Old Yellow Enzymes (OYEs, EC 1.6.99.1) are a class of flavin-dependent ene-reductases (ERs) catalyzing the asymmetric hydrogenation of electronically activated C=C bonds in the presence of nicotinamide cofactors. We have identified and produced four new putative ERs from the filamentous fungi Aspergillus niger CBS 513.88 and Botryotinia fuckeliana B05.10. Based on the most recent classification, AnOYE2 and BfOYE1 belong to Class II OYEs, as they share all the fingerprint motifs described for “classical” OYE homologues identified in fungi. On the other hand, AnOYE8 and BfOYE4 share most of the typical conserved residues reported in Class III OYEs (S23, P24, C26, A60, Q102, R215, S249, Q265, G284, M285, F305, G307, R308, and R312; YqjM numbering).

AnOYE8 was solved and refined in the C121 space group with four molecules per asymmetric unit. The overall structure of a single subunit showed the typical conserved α8/β8-TIM barrel fold. In agreement with the general behavior of Class III OYEs, the four molecules within the asymmetric unit assembled into dimers with the functional quaternary architecture peculiar of these enzymes. AnOYE8 is an elongated dimer composed of two protomers with an interacting surface of 2807 Å2 (data obtained by EMBL-EBI-PISA analysis). Both the α1-helix and loop 3 (capping subdomain), as well as the peculiar long N-terminal and C-terminal loops of each protomer, were involved in the dimerization surface, which contained 71 interfacing residues that established 18 hydrogen bonds and 8 salt bridges. The C-terminus of each subunit (from Gly393 to Lys416) protruded through an “amino acid finger” (Trp397) that reached the active site of the adjacent subunit, shaping the entrance and the catalytic cavity of each subunit. AnOYE8 accommodated a non-covalently bound FMN cofactor molecule lying at the bottom of the active site pocket. Similar to other Class III OYEs, AnOYE8 contained the highly conserved proton donor Tyr220 and the histidine pair (His215 and His218) involved in the binding and proper orientation of the substrate through hydrogen bonding with the electron-withdrawing group of the substrate. The omit electronic density map revealed the presence of a small organic molecule, most likely SO4 anion, present within the crystallization precipitant agents, lying on top of the isoalloxazine ring of FMN. In the complex with SO4, two oxygens of the compound formed two hydrogen bonds with the side chain of His215 and Tyr220, thus confirming the importance of these residues in substrate orientation and catalysis.

>[4x]MKDIKVEPAKGISYFTPAQETPAGTAANPQTSGKAIPKLFQPITIRGLTFQNRLGVSPMCQYSAEDGHMTDYHLAHLGGIAQRGPGLIMIEATAVQPEGRISPQDVGLWKDSQIAPIARVIEFAHSQGQKIGIQLAHAGRKASTTVPWMLNHGSIATENVGGWPDNVKGPSDIPFSETFPRPRAMTQDDIREFKEAWVAAAKRALVAGADFIEIHNAHGYLLASFLTPYANKRTDEYGGSFENRMRLPLKIAQLTRDTVGEHVPVFLRLSASDWLGSTSTETWDLQHAVRFAEALADQGAIDLVDVSSGGLHSSQEVKSGPGFQAPFGIAVKKAVGERMLVATVGHIRDGKLANRLLEEEGLDVVLVGRGFQKDPGLVWTFAQHLDVEVAMPGQIRWGFSKQGRRGTPFVDPSVYKPSVIEP Deubiquitinating enzymes (DUBs) cleave peptide- and isopeptide-bonds downstream of ubiquitin. By performing a comprehensive bioinformatical screen, followed by biochemical and structural characterization of interesting candidates, we were able to identify active members of this family in a wide range of eukaryotic species and a few host-associated bacteria. Due to the similarity to the herpesvirus proteins, we refer to this extended enzyme family as VTD (for Viral Tegument-like Deubiquitinases). While some VTD activities resemble viral tegument DUBs in that they favor K48-linked ubiquitin chains, other members are highly specific for K6- or K63-linked ubiquitin chains.

In the di-ubiquitin cleavage assay, Wc-VTD1 showed a strong preference for K6-linked chains. In order to gain insight into the functional differences of bacterial VTDs in comparison to their relatives from viruses and transposons, the structure of Wc-VTD1 was solved in the unbound form at 1.8 Å resolution as well as in a covalent complex with ubiquitin at 1.9 Å resolution. The tertiary structure contains nine α-helices and seven β-strands, adopting a fold with overall similarity to the viral and transposon-encoded VTDs. The catalytic triad is formed by Cys319, Asp440, and His442. As previously observed in the M48 crystal structure, the conformation of the catalytic histidine appears as non-productive for catalysis due to the large distance to the cysteine. The structures in the unbound and complexed state can be superimposed with an RMS distance of 0.538 Å over 144 Cα-atoms excluding some 40 residues, thus indicating little overall conformational changes upon binding to the Ub-PA substrate. On the opposite side, helix α1 (residues 302 to 305) together with the following amino acids 306 to 311 is also shifted by a distance of about 8 Å. However, helix α1 itself does not seem to be involved in direct interactions with the bound substrate. It is located on the surface rather distant from the active site and is involved in the crystal contacts between the two crystallographically independent molecules in the apo structure. In fact, the available structure and mutagenesis data suggest an attractive three-step model for explaining the K6 specificity of Wc-VTD1: In the apo-form, the α1 and α9 helices are far apart and the catalytic histidine residue is in a non-productive conformation.

>[2x]KMPEEEQDSLAAFSRIEANITQYDPLLDNAGKSACTCICLKAAEMLLEASPDQVNAGLIDDILVEGVADYNRFKVGGVVEHTSVENYELNTFELKRLEFRDVDNPFSAEGNPYAGTLDSFAKMMEKASDSKDLPKPVALVMTKSNMTITIVIRPDGKYWLFDPHGTNGKGAYIESCNTDELIKKIKEIFPKTSYPGMTEDENLGFNSFEAYAVRR> XPCYE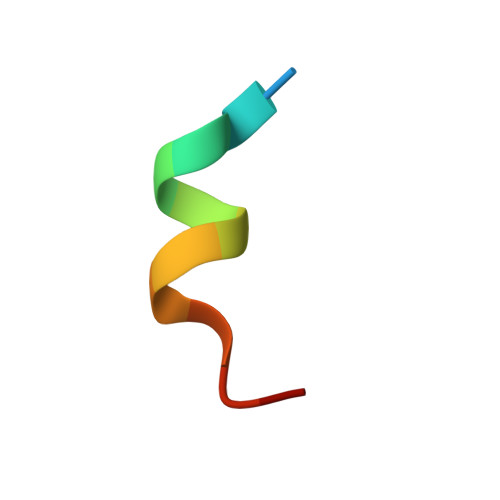AWVLCEYX SAP05 binds both the von Willibrand factor type A (vWA) domain of Rpn10 and the zinc-finger (ZnF) domain of multiple members of two distinct plant transcription factor families, known as SQUAMOSA-PROMOTER BINDING PROTEIN-LIKE (SPL) and GATA BINDING FACTORS (GATAs). The SAP05 protein comprises a globular compact structure with five β-strands that form an internal triangular mixed β-sheet core. β-strand 1 (β1) locates on the long end of this triangular core and connects via a loop–helix–loop–helix–loop structure to β2 at the opposite surface near the tip of this core. The SAP05 residues binding ZnF and vWA are located at opposing surfaces of the effector with the ZnF binding surface comprising the loop-dominated surface (loop surface) and the vWA-binding surface the β-sheet-dominated long end of the triangular β-sheet core (sheet surface). Our data show how the bacterial SAP05 effector has evolved as a functional adapter of the 26S proteasome to bypass the canonical UPS cellular proteolysis pathway and enable ubiquitin-independent degradation of structured eukaryotic proteins.

The crystal structure contains eight copies of the 1:1 complex in the asymmetric unit (ASU), which are closely similar. In addition to the two structural Zn2+ ions within each SPL5ZnF domain, a further four Zn2+ ions are found in the ASU forming crystal contacts. These involve E80 from four of the eight SAP05 molecules and H82 and E118 from separate neighbouring copies of SPL5ZnF. The SAP05 loop surface that interacts with ZnF comprises three distinct protruding loops that are separated by β-strands and involves six amino acids of which D66 locates in loop 4, G76, N77, and E80 in loop 5, and R104 and D106 in loop 7 of the SAP05 structure. SAP05 binds the two SPL5 ZnF sites, which are held together by Zn2+ ions and the complex involve nine connections, with SAP05 amino acids N77 interacting with three amino acids, D106 with two and SAP05 D66, G76, E80, and R104 each with one amino acid of SPL5ZnF, and SAP05 E80 and D106 each forming two interactions with R81 and R121, respectively, of SPL5ZnF. The majority of the interactions are mediated by hydrogen bonds with some salt bridges and are reinforced by nonbonded contacts. The SAP05–ZnF interaction is dominated by electrostatic interactions of charged and polar residues at the SAP05 loop surface and oppositely charged or polar residues located within α-helices of SPL5ZnF. Titration of SAP05 into a solution of SPL5ZnF showed an exothermic binding isotherm with a fitted dissociation equilibrium constant (Kd) of 0.45 ± 0.06 µM and stoichiometry of 1:1, and titrating SPL5ZnF into a solution of SAP05 showed a Kd of 0.52 ± 0.05 µM. Therefore, D66, N77, and D106 are required for the SAP05 interactions with the ZnF domain of SPLs. Taken together, these results indicate that the electronegative surface potential contributed by D66 is an important factor for binding SPL and GATA TFs.

>[8x]GPAPNEEFVGDMRIVNVNLSNIDILKKHETFKKYFDFTLTGPRYNGNIAEFAMIWKIKNPPLNLLGVFFDDGTRDDEDDKYILEELKQIGNGAKNMYIFWQYEQK;>GPSRLCQVDRCTVNLTEAKQYYRRHRVCEVHAKASAATVAGVRQRFCQQCSRFHELPEFDEAKRSCRRRL[8x]>[4x]SNAMTNVLYQHGTLGTLMAGLLEGTATINELLEHGNLGIATLTGSDGEVIFLDGKAYHANEHKEFIELKGDEKVPYASITNFKASKTFPLQQLSQDDVFA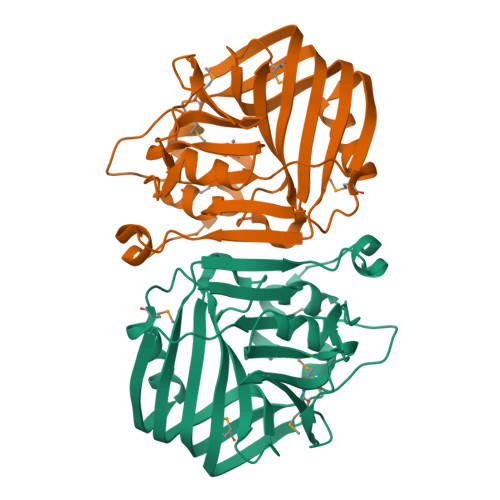QIKNEMLSENLFSAVKIYGTFKHMHVRMMPAQQPPYTRLIDSARRQPEEKRQDIRGAIVGFFTPELFHGVGSAGFHIHFADDERAYGGHVLDFEVDDVVVEIQNFETFQQHFPVNNETFVKAKIDYKDVAEEIREAE>MARTVVLITGCSSGIGLHLAVRLASDPSQSFKVYATLRDLKTQGRLWEAARALACPPGSLETLQLDVRDSKSVAAARERVTEGRVDVLVCNAGLGLLGPLEALGEDAVASVLDVNVVGTVRMLQAFLPDMKRRGSGRVLVTGSVGGLMGLPFNDVYCASKFALEGLCESLAVLLLPFGVHLSLIECGPVHTAFMEKVLGSPEEVLDRTDIHTFHRFYQYLAHSKQVFREAAQNPEEV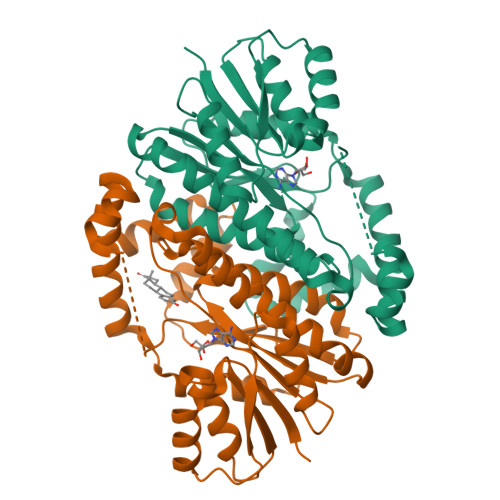AEVFLTALRAPKPTLRYFTTERFLPLLRMRLDDPSGSNYVTAMHREVFGDVPAKAEAGAEAGGGAGPGAEDEAGRGAVGDPELGDPPAAPQ[2x]>[2x]GHIKQLLKNKRFEVIKALVESKKIKQEWLEDLYSILLKQDTDVEITQAKYEIIKLLLTEKKYLNFELLTKTLNLDQQTAIEIMRNPFKEVYFPTYNIENPEESRLNKALIIPLSNQTFTLNTFVNSQDLETIKEATNKNFFVIFDNIFSGKSYQLAVAAGLIAKEKEILDNVAFTGEVSSNGFIIPVNHLEEKKEITEKAKKVLITPEDIENLEELSFWLNPEHLPVIFIHINKPELALQSLKQMEDAIKKDERFKYFKLENLKKFYRLEDQDMYLITPSVDFSNREELIKILNEFREKVSKLLTLEGVIKDHNKVVLNISAGISTLALYFGVILGNRQASIIYHYQKEYHKVIDLTDNPRKIKEKKSEFEKISVNKNIQDPLMIIIYLASHNPIEKGLELKEKLRAKGELIIQSKEHQGNLEIGDWSDIVSEIYTAIDDNKQKENYMVFSAPVAIMLALGMALGYFLPIKVFHYNRDEYIEVP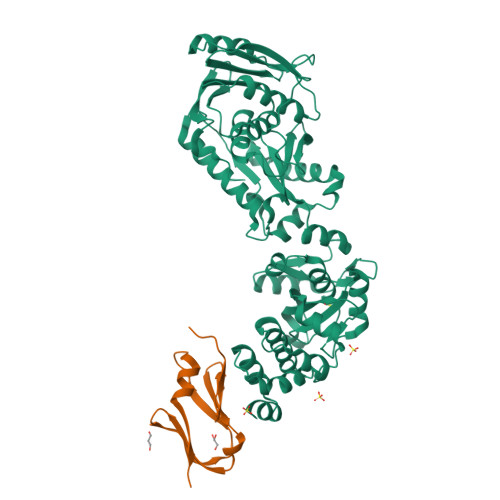IKLNEEILRSPF;>STSQKATYTDDFVLYRGDDFIEIIIDEKYLNKKVKILLDNDTIFNGILKDTSIFIPVKEQIDLEELAKHISILPEG[2x]> MATRLDRLVTILETGSTRLIRDTAVNQLADWQKQHPEELFNLLSRVVPYLRHKDWETRTTAAKAIGKIIENAPLYDPNAGQDEAAPEPTNGSFEVKKEEEKDVLEQDNFFRLESLDVATIVKYGRPLLRGGPVDYNLAALDPQKRLAHLKKTLNGRLGLLGRVFEDEEMPVEQIASPITPNDAAGANGVGRQDGASNDNQSQAIDESKMSARQLNVLKRKRKREAQKAAQGKSGFGDLSLRRSTTAGSDAFGEDTPMPDADSKKNKLAEYFSLDRP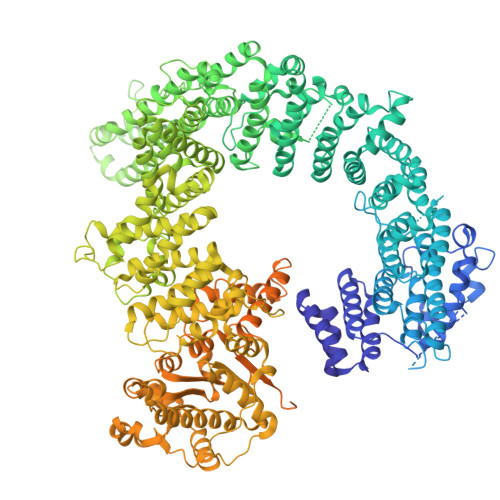ENTEEDTKIVSEFKGPVLPIKSEIEADDSLEGAEWPFERLCEFLKVDLFDPQWETRHGAAMGLREVIRVHGAGAGRRRGKTRKENNDLNRQWLDDLAYRLLCVLMLDKFTDYSSDTSVAPIRETVGQTLGAVLRHISVESVHAIYRLLYCMVTQEDLPSEQNMWAVCHGGMVGLRYVVAVRKDLLLQDGDMIDGVVRCVMQGLGDIDDDVRSVSAATLIPMAKEFVMMRRSALDSLINIVWESLSNLGDDLSASTGKIMDLLATLCSFPEVLEAMKVSASQDEERSFTLLVPRLYPFLRHTITSVRLAVLKALMTFANLGGETSQGWLNGRILRLIFQNIIVERDQDTLNMSLELWTTLVRRLAARDPAILADEFEAHAEPMMQLALHPIGVPRHPIPMNPALFQKPSGGTYSLPGASQTNSRRSSPPEGERATKRRRKSTKAEDVAPSTHTHDVDGHMIQGEVDLVGVDVLIRSRISAAKAMGLIMSFIPTPRLASYDTAVLQALSSPYASTQLAAAMVIDEYAKNCSTPEVASRFIEPLQKIIDLERPSHYRDLVTYVQRVRSASQQLINLFRDHGKVSQGKLPTLAVVVQGEPEAGPGAFSIANAEKVVNEDFERLKRLMAPGQRLIALPQLNEAREQTVEVIEEAKAAKEARDARIKAAAACALVAMKVLPKKPSPLIKAIMDSIKTEENQELQSRSAATIARLVQLFTESGRRGPAEKVVANLVKFSCVEVAETPEFPIHAHKTNVILSMQKEEDRVDHPDAVKYAREAKAARITRRGAKEALEILSKNFGAELLERVPTLRTFMEEPLVRAFSGDLPPEARDPENAFGQEIVDAMSVIRTMTPTLHPALHPFVMQQVPLVIKALRSDLSVFRYMAAKCMATICSVITVDGMTALVEKVLPSINNPLDLSFRQGAIEVIYHLIAVMGDAILPYVIFLIVPVLGRMSDSDNQIRLIATTSFATLVKLVPLEAGIPDPPGLSEELLKGRDRERTFIAQLLDPKKIEPFKIPVAIKAELRSYQQEGVNWLAFLNKYHLHGILCDDMGLGKTLQTICIVASDHHQRAEEFARTGAPEVRKLPSLIICPPTLSGHWQQEIKTYAPFLTVTAYVGSPAERRAMKDSLDKTDIVITSYDVCRNDIDVIEKYNWNYCVLDQGHLIKNPKAKITLAVKRLTSNHRLILTGTPIQNNVLELWSLFDFLMPGFLGAEKVFLDRFAKPIANSRYSKASSKEQEAGALAIEALHKQVLPFLLRRLKEEVLNDLPPKILQNYYCDLSDLQRKLFEDFTKREGKKITETAGRDDKEAKQHIFQALQYMRKLCNSPALVMKPGHKAYEDTQKYLAKHGTTLEDPIHAPKLGALRDLLVDCGIGVEGQESSDPLYTPIKPHRALIFCQMKEMLDMVQNTVLKQMLPSVSYLRLDGSVEANKRQDIVNKFNSDPSYDVLLLTTSVGGLGLNLTGADTVIFVEHDWNPQKDLQAMDRAHRIGQKKVVNVYRIITRGTLEEKILSLQRFKIDVASTVVNQQNAGLATMDTDQILDLFNLGESGPSLITDNKESIEGREEDMVDIETGDVRRPGKKAAWLEGLGELWDNAQYEESFDLDGFLKTMQAAAWSHPQFEK>[60x]MGSSHHHHHHSSSAALEVLFQGPAPEDLLERLLGEMELELIELRRALAQTIATFKSTERQRDAQQLIAQRWYEKAQAALDRGNEQLAREALGQRQSY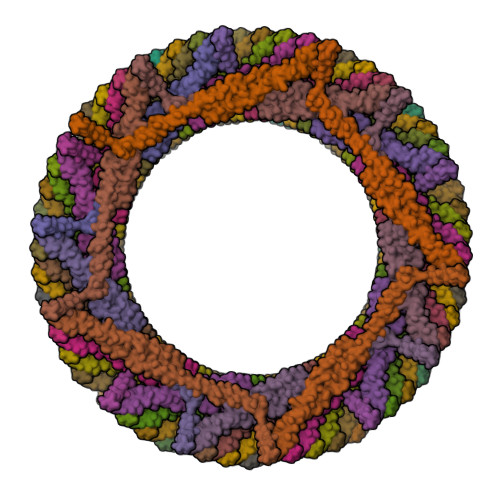QSHTEALGKSLGEQRALVEQVRGQLQKLERKYLELKSQKNLYLARLKSAIAAQKIEEIAGNLDNASASSLFERIETKILELEAERELLNPPPSPLDKKFEQWEEQQAVEATLAAMKARRSLPPPSS> SHMSELSEIDSVAGVTIYSVDGEPKSFVYKAGFAIDADGAPNAYAPNNGGTDFTANGGDDQGGDWWGGPVDAEGYPIKQKIFDPFPGYYVSATAHFNPAYSEDSPYRYIDSNSIPFIVLPGNHSNGAKLGDVALVYNEKTGDNCYAIYGDVGPSSKIGQGSVRLAQALKIDDNPKAGGTESRIVVTLVFPGSVGKWETPKRWFSHANQLTKAWGGLSRLKTLSDQL

We focus on AMGs that potentially encode chitosanase enzymes that metabolize chitin – a common carbon polymer. One expressed protein showing endo-chitosanase activity (V-Csn) is crystalized and structurally characterized at ultra-high resolution, thus representing the structure of a soil viral AMG product. The structure consisted of two non-contiguous structural domains. Our rigorous analyses not only resulted in a crystal structure of a soil viral AMG product, but also enabled us to propose the mode of action of this previously uncharacterized chitosanase enzyme in the GH75 family of glycosyl hydrolases.

Based upon a partial alignment of the V-Csn, A. fumigatus, F. solani, and S. avermitilis sequences, the corresponding residues in V-Csn are D148 and E157. Two V-Csn constructs harboring either a D148N substitution or a E157Q substitution were generated, and the activities of the respective mutant enzymes measured. Activity was reduced five-fold for D148N and almost eliminated for E157Q. Both constructs eluted with gel-filtration chromatography retention times identical to native V-Csn, and circular dichroism spectra indicated both constructs were folded. In both cases the carboxylate was converted to the corresponding amide, generating the mutant proteins D148N and E157Q. The two mutant V-Csn proteins were crystallized under the same conditions as the wild-type protein, and their structures were determined by molecular replacement to high resolution. Superposition of the two mutant structures onto the wild-type apo1 structure gave RMSDs of 0.11 and 0.07 Å, respectively, for all Cα positions, suggesting very little conformational differences between the mutant and the wild-type structures. Structural data from Cel45 and CaCel45 suggest that this acidic residue is the catalytic proton donor in the GH45 enzymes, and given the structural similarity of the DPBB domains in the GH45 and GH75 enzymes, it is highly likely that E157 is the catalytic proton donor in V-Csn.> VSIYDPAAADRAEEERIERWVEQLREALVGDGFLLHYQPVLNLQGEPLELYQAFLRLERNGEMMSPNAFMAIAEEHDLVTEIDRWVVARAIRQLGERQRAGHKTHLLVRIGPNSFSDPQMIDTIREQLAVYGVPGERLWLQTPESKVFTHLRNAQQFLAAVSAMDCKVGLEQFGSGLDSFQLLAHFHPAFLKLDRGITGDIASARDSQEKIREITSRAQPAGILTMAEFVADAQSMSSFFSAGVDYVQGDFVA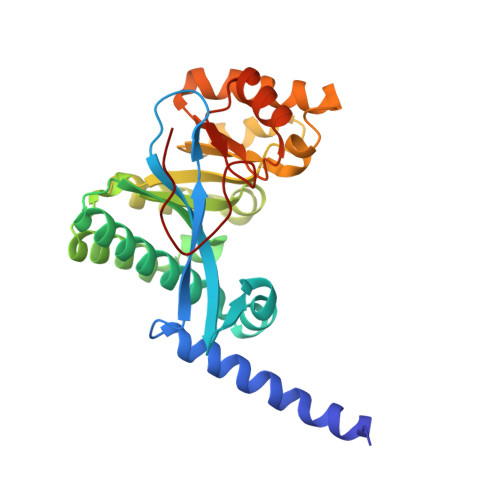PTGPLMNYEFG> GSMVEATAQETDRPRFSFSIAAREGKARTGTIEMKRGVIRTPAFMPVGTAATVKALKPETVRATGADIILGNTYHLMLRPGAERIAKLGGLHSFMGWDRPILTDSGGYQVMSLSSLTKQSEEGVTFKSHLDGSRHMLSPERSIEI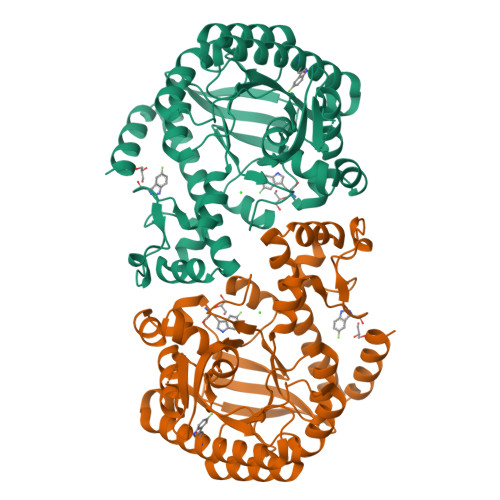QHLLGSDIVMAFDECTPYPATPSRAASSMERSMRWAKRSRDAFDSRKEQAENAALFGIQQGSVFENLRQQSADALAEIGFDGYAVGGLAVGEGQDEMFRVLDFSVPMLPDDKPHYLMGVGKPDDIVGAVERGIDMFDCVLPTRSGRNGQAFTWDGPINIRNARFSEDLKPLDSECHCAVCQKFSRAYIHHLIRAGEILGAMLMTEHNIAFYQQLMQKIRDSISEGRFSQFAQDFRARYFARNS> MTRYYCEYCHSYLTHDTLSVRKSHLVGKNHLRITADYYRNKARDIINKHNHKRRHIGKRGRKERENSSQNETLKVTCLSNKEKRHIMHVKKMNQKELAQTSIDTLKLLYDGSPGYSKVFVDANRFDIGDLVKASKLPQRANEKSAHHSFKQTSRSRDETCESNPFPRLNNPKKLE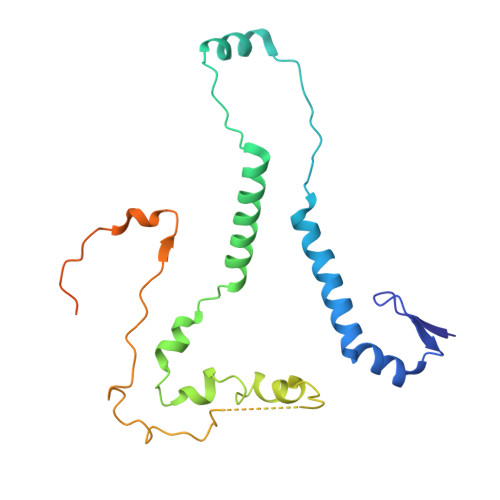PPKILSQWSNTIPKTSIFYSVDILQTTIKESKKRMHSDGIRKPSSANGYKRRRYGN> SSQIRQNYSTEVEAAVNRLVNLYLRASYTYLSLGFYFDRDDVALCGVCHFFCELAEEKREGAERLLKMQNQRGGRALFQDLQKPSQDEWGTTLDAMKAAIVLEKSLNQALLDLHALGSAQADPHLCDFLESHFLDEEVKLIKKMGDHLTNIQRLVGSQAGLGEYLFERLTLKHD

Among various protein templates, the self-assembled 24-mer protein cage of ferritin is of particular interest as it is naturally designed for iron storage. Using this concept, we replaced the Glu45 and Arg52 residues of recombinant L-chain apo-Fr from horse liver (apo-rHLFr) by Cys and the resulting apo-rHLFr mutant apo-E45C/R52C-rHLFr was used in the current study. Herein we describe a crystal structure analysis of Au(III) ions accumulated in the ferritin cage and subsequent reduction of the metal ions by sodium borohydride inside the crosslinked single crystal. In summary, we have demonstrated structural evidence for the formation of an Au sub-nanocluster inside the narrow three-fold symmetric channel of the apo-ferritin cage.

The structure of the crosslinked crystal (Au·CL-apo-E45C/R52C-rHLFr) was refined to 1.95 Å resolution. The root-mean-square deviation of the Cα atoms of Au·CL-apo-E45C/R52C-rHLFr from that of apo-rHLFr is 0.25 Å. This indicates that the folding of apo-rHLFr is preserved even after the accumulation of Au(III) ions and the crosslink treatment. All of the Au binding sites in the ferritin cage are divided into three deposition regions; the three-fold axis channel (Site-A), the metal accumulation site (Site-B) and at Met96 (Site-C). At Site-A, there are two Au atoms, one of which (Au1) is coordinated by Cys126 and a water molecule. The other Au ion (Au2) at Site-A is coordinated by both His114 and Cys126. Cys126 forms a bridge between Au1 and Au2, giving Au–Sγ(Cys) distances of 2.39 and 2.26 Å, respectively. At Site-B, three different Au ions (Au3–Au5) are present, which form a thiol-bridged (Cys48 and Cys52) trinuclear structure. At Site-C, Au6 and Au7 are coordinated by His147 and Met96. Although the total number of Au binding sites observed from the crosslinked crystal is 192, the sum of Au atoms estimated from all of the occupancies is 96, which is consistent with that obtained from the quantitative analyses (ICP/BCA) (107±4).> GSD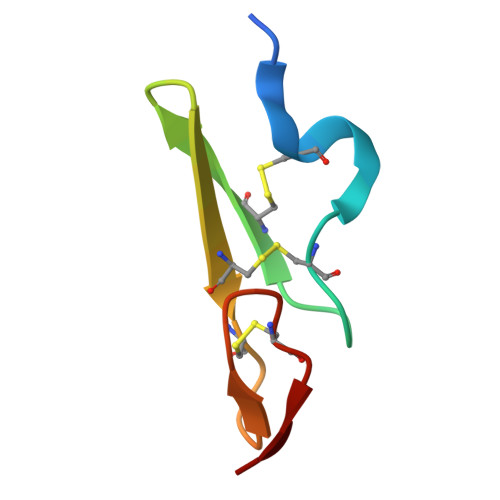VNECVSNPCQNDATCLDQIGEFQCICMPGYEGVHCEVNT N-[2-(diethylamino)ethyl]-5-[(Z)-(5-fluoro-2-oxo-1,2-dihydro-3H-indol-3-ylidene)methyl]-2,4-dimethyl-1H-pyrrole-3-carboxamide | C22 H27 F N4 O2 | 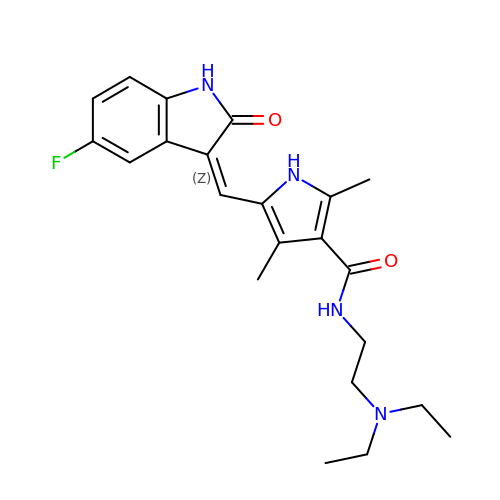WINHZLLDWRZWRT-ATVHPVEESA-N> MTTNDTYEATYAIPMHCENCVNDIKACLKNVPGINSLNFDIEQQIMSVESSVAPSTIINTLRNCGKDAIIRGAGKPNSSAVAILETFQKYTIDQKKDT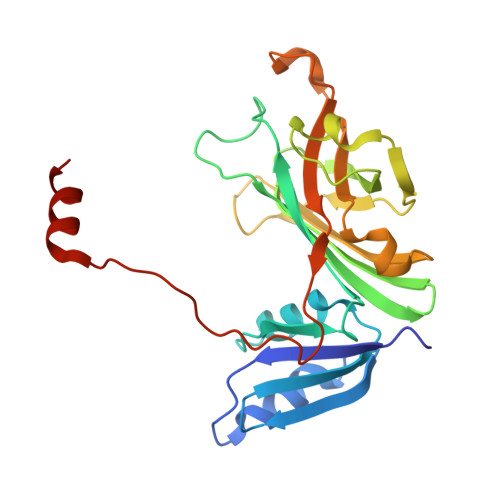AVRGLARIVQVGENKTLFDITVNGVPEAGNYHASIHEKGDVSKGVESTGKVWHKFDEPIECFNESDLGKNLYSGKTFLSAPLPTWQLIGRSFVISKSLNHPENEPSSVKDYSFLGVIARSAGVWENNKQVCACTGKTVWEERKDALANNIK> EEIIWESLSVDVGSQGNPGIVEYKGVDTKTGEVLFEREPIPIGTNNMGEFLAIVHGLRYLKERNSRKP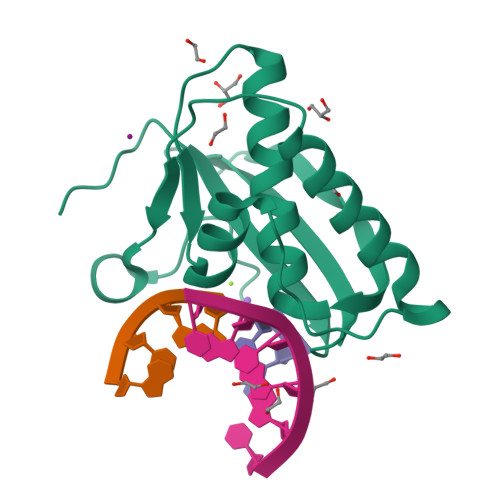IYSDSQTAIKWVKDKKAKSTLVRNEETALIWKLVDEAEEWLNTHTYETPILKWQTDKWGEIKADYGR NOGALAMYCIN | C39 H49 N O16 | 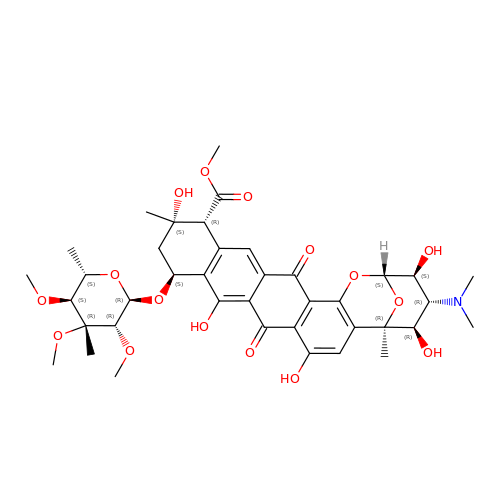KGTDRFCXGRULNK-JYOBTZKQSA-N>[2x]GPLVLIGSGLSSEQQKMLSELAVILKAKKYTEFDSTVTHVVVPGDAVQSTLKCMLGILNGCWILKFEWVKACLRRKVCEQEEKYEIPEGPRRSRLNREQLLPKLFDGCYFYLW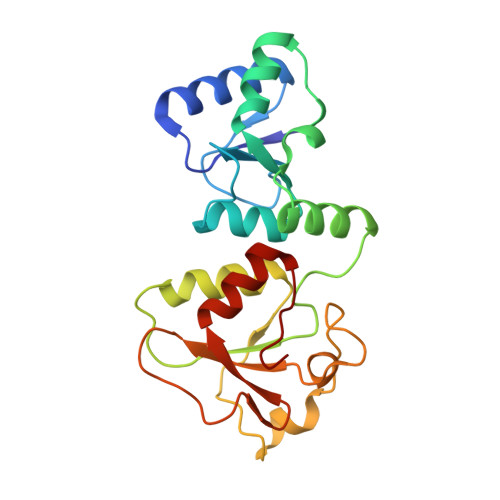GTFKHHPKDNLIKLLTAGGGQILSRKPKPDSDVTQTINTVAYHARPDSDQRFCTQYIIYEDLCNYHPERVRQGKVWKAPSSWFIDCVMSFELLPLDS>[3x]MFEARLVQGSILKKVLEALKDLINEACWDISSSGVNLQSMDSSHVSLVQLTLRSEGFDTYRCDRNLAMGVNLTSMSKILKCAGNEDIITLRAEDNADTLALVFEAPNQEKVSDYEMKLMDLDVEQLGIPEQEYSCVVKMPSGEFARICRDLSHIGDAVVISCAKDGVKFSASGELGNG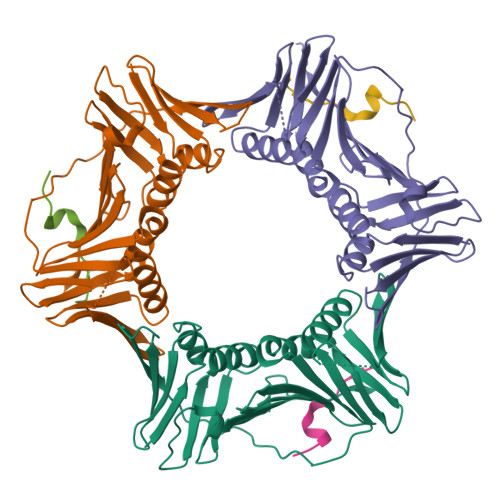NIKLSQTSNVDKEEEAVTIEMNEPVQLTFALRYLNFFTKATPLSSTVTLSMSADVPLVVEYKIADMGHLKYYLAPKIEDEEGS;>KANRQVSITGFFQRK[3x]> PISPIETVPVKLKPGMDGPKVKQWPLTEEKIKALVEICTEMEKEGKISKIGPENPYSTPVFAIKKKDSTKWRKLVDFRELNKRTQ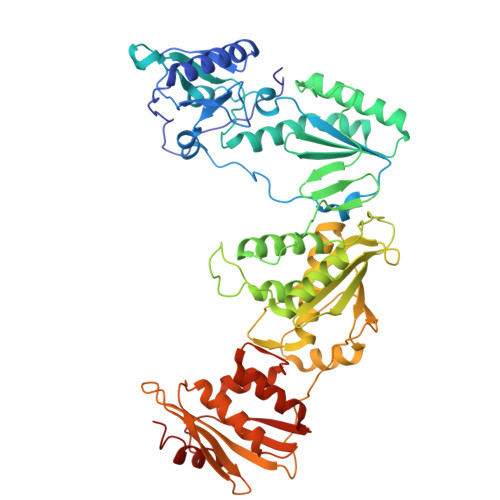DFWEVQLGIPHPAGLKKKKSVTVLDVGDAYFSVPLDEDFRKYTAFTIPSINNETPGIRYQYNVLPQGWKGSPAIFQSSMTKILEPFKKQNPDIVIYQYMDDLYVGSDLEIGQHRTKIEELRQHLLRWGLTTPDKKHQKEPPCLWMGYELHPDKWTVQPIVLPEKDSWTVNDIQKLVGKLNWASQIYPGIKVRQLCKLLRGTKALTEVIPLTEEAELELAENREILKEPVHGVYYDPSKDLIAEIQKQGQGQWTYQIYQEPFKNLKTGKYARMRGAHTNDVKQLTEAVQKITTESIVIWGKTPKFKLPIQKETWETWWTEYWQATWIPEWEFVNTPPLVKLWYQLEKEPIVGAETFYVDGAANRETKLGKAGYVTNKGRQKVVPLTNTTNQKTQLQAIYLALQDSGLEVNIVTDSQYALGIIQAQPDKSESELVNQIIEQLIKKEKVYLAWVPAHKGIGGNEQVDKLVSAGIRHHHHH>MVSKGEELIKENMHMKL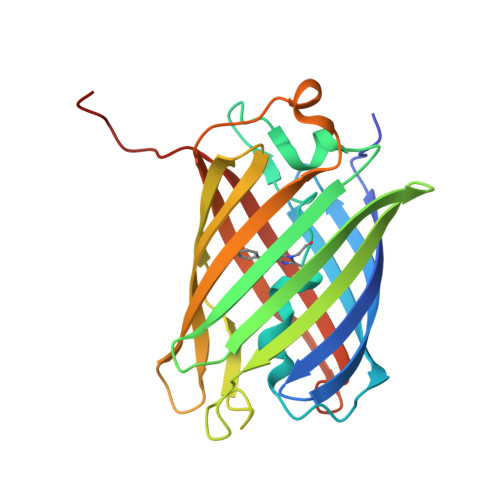YMEGTVNNHHFKCTSEGEGKPYEGTQTMRIKVVEGGPLPFAFDILATSFMYGSRTFINHTQGIPDFFKQSFPEGFTWERVTTYEDGGVLTATQDTSLQDGCLIYNVKIRGVNFPSNGPVMQKKTLGWEANTEMLYPADGGLEGRSDMALKLVGGGHLICNFKTTYRSKKPAKNLKMPGVYYVDHRLERIKEADKETYVEQHEVAVARYCDLPSKLGHKLN[4x]> MQPPVANFCLWNLQPIQGSWMGAACIYQMPPSVRNTWWFPLLNTIPLDQYTRIYQWFMGVDRDRSGTLEINELMMGQFPGGIRLSPQTALRMMRIFDTDFNGHISFYEFMAMYKFMELAYNLFVMNARARSGTLEPHEILPALQQLGFYINQRTSLLLHRLFARGMAFCDLNCWIAICAFAAQTRSAYQMIFMNPY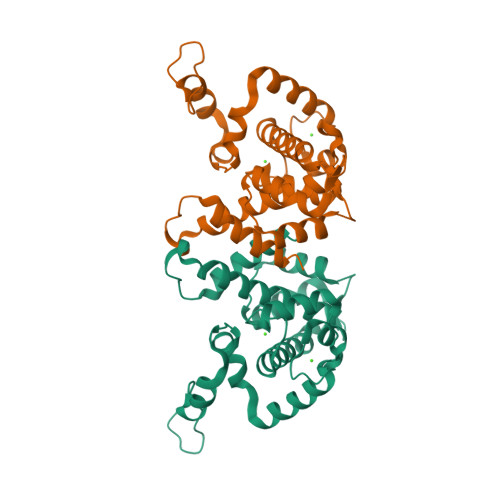YGPMKPFNPMEFGKFLDVVTSLLE>GILELAGTVGCVGPRTPIAYMKYGCFCGLGGHGQPRDAIDWCCHGHDCCYTRAEEAGCSPKTERYSWQCVNQSVLCGPAENKCQELLCKCDQEIANCLAQTEYNLKYLFYPQFLCEPDSP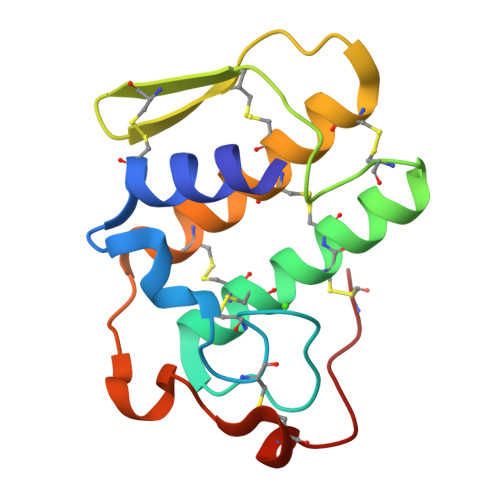KCD[3x]>STEAQEGVIKVATQSETVTGTSANTAVSPKNLKWIAQSEPTWAATTAIRGFVKTSSGSITFVGNDTVGSTQDLELYEKNSYAVSPYELNRVLANYLPLKAKAADTNLLDGLDSSQFIRRDIAQTVNGSLTLTQQTNLSAPLVSSSTGEFGGSLAANRTFTIRNTGAPTSIVFEKGPASGANPAQSMSIRVWGNQFGGGSDTTRSTVFEVGDDTSHHFYSQRNKDGNIAFNINGTVMPININASGLMNVNGTATFGRSVTANGEFISKSANAFRAINGDYGFFIRNDASNTYFLLTAAGDQTGGFNGLRPLLINNQSGQITIGEGLIIAKGVTINSGGLTVNSRIRSQGTKTSDLYTRAPTSDTVGFWSIDINDSATYNQFPGYFKMVEKTNEVTGLPYLERGEEVKSPGTLTQFGNTLDSLYQDWITYPTTPEARTTRWTRTWQKTKNSWSSFVQVFDGGNPPQPSDIGALPSDNATMGNLTIRDFLRIGNVRIVPDPVNKTVKFEWVE[3x]

The proximal half-fiber is formed by a parallel homo-trimer of gp34. The protein is a highly intertwined trimer containing a 2 nm-wide triple β-helix domain interspersed with three wider domains in which each of the monomers forms an anti-parallel β-sheet. The long tail fibers recognize the outer membrane protein C (OmpC) or the lipopolysaccharide (LPS) of E. coli and are responsible for the initial and reversible attachment of the virion. The carboxy-terminal parts of gp34 that we crystallized occupy the part of the proximal tail fiber closest to gp35 (the “knee”).

Crystals of gp34(781–1289) and gp34(726–1289) also belong to space group P21, but with different cell parameters. The structures of gp34(781–1289) and gp34(726–1289) were also solved by molecular replacement, both with one trimer in the asymmetric unit and belonging to the P21 space group. After manual adjustments and refinement, the gp34(781–1289) structure contained 1485 residues (795–1289 in each of the three chains), plus 3 phosphate ions, 17 glycerol molecules, 1822 water molecules, three phosphate ions, a urea molecule, and two acetate ions. Note that this structure contains selenomethionine residues instead of methionine, although these were not used for phasing. The N-termini of gp34(726–1289) and gp34(781–1289) are less well ordered in the crystal structures, presumably due to flexibility and lack of crystal contacts in these regions. Residues 796–878 form two domains, each with three central short α-helices decorated by intertwined loops. They are followed by a triple-helical neck and a stretch of residues in which two turns are present. In the repeat consisting of residues 822–868, the non-conserved loop (amino acids 837–859) points upwards, forming a 2-nm long β-hairpin lying against the three-helix bundle. The extensive intertwining of the three monomers in the trimer leads to a large fraction of buried monomer surface in the trimer, a large amount of inter-molecular hydrophobic and polar interactions, and thus a very high energy barrier to dissociation. This predicted stability is consistent with the observed heat and protease stability of gp34(781–1289).> MENTENSVDSKSIKNLEPKIIHGSESMDSGISLDNSYKMDYPEMGLCIIINNKNFHKSTGMTSRSGTDVDAANLRET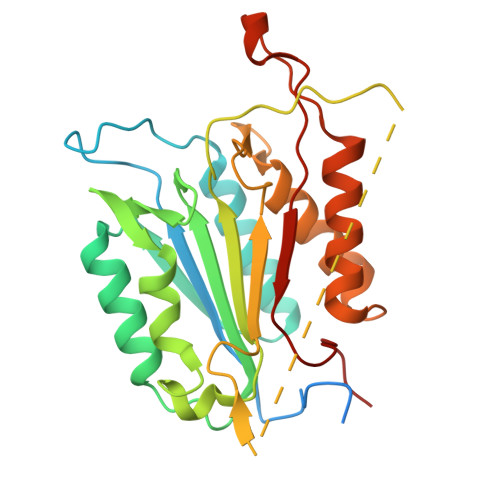FRNLKYEVRNKNDLTREEIVELMRDVSKEDHSKRSSFVCVLLSHGEEGIIFGTNGPVDLKKITNFFRGDRCRSLTGKPKLFIIQACRGTELDCGIETDSGVDDDMACHKIPVEADFLYAYSTAPGYYSWRNSKDGSWFIQSLCAMLKQYADKLEFMHILTRVNRKVATEFESFSFDATFHAKKQIPCIDSMLTKELYFYHL> GPKPKNTKENLSKSSWRQEWLANLKLISVSLVDEFPSELSDSDRQIINEKM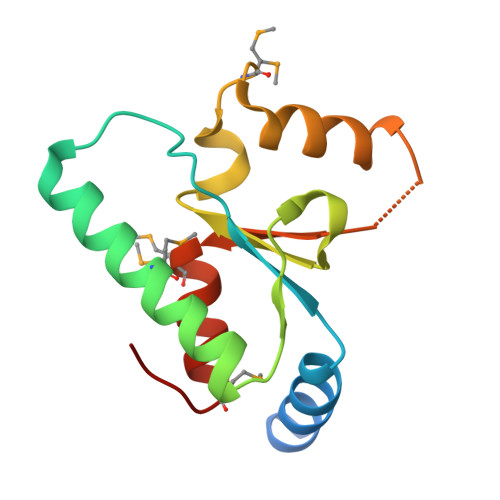QLLKDIFANNLKSAISNNFRESDIIILKGEIEDYPMSSEIKIYYNELQNKPDAKKARFWSFMKTQRFVSNMGFDIQ> IVGGYTCGANTVPYQVSLNSGYHFCGGSLINSQWVVSAAHCYKSGIQVRLGEDNINVVEGNEQFISASKSIVHPSYNKRRKNNDIMLIKLKSAASLNSRVASISLPTSCASAGTQCLISGWGNTKSSGTSYPDVLKCLKAPILSDSSCKSAYPGQITSNMFCAGYLEGGKDSCQ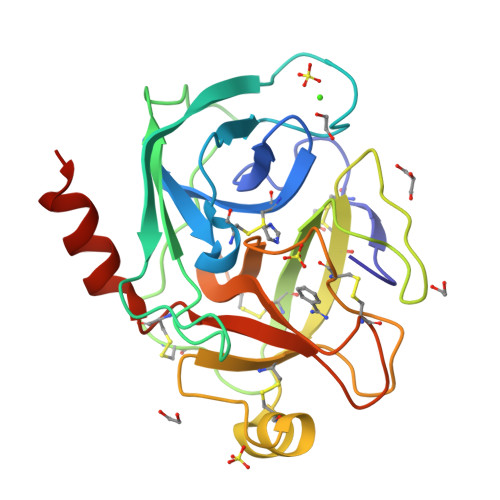GDSGGPVVCSGKLQGIVSWGSGCAQKNKPGVYTKVCNYVSWIKQTIASNHHHHHH>[3x]ARASPGSAASPRLREGPELSPDDPAGLLDLRQGMFAQLVAQNVLLIDGPLSWYSDPGLAGVSLTGGLSYKEDTKELVVAKAGVYYVFFQLELRRVVAGEGSGSVSLALHLQPLRSAAGAAALALTVDLPPASSEARNSAFGFQGRLLHLSAGQRLGVHLHTEARARHAWQLTQGATVLGLFRVTPEIPAGLPSPRSEGSHHHHHHHH;>[3x]QDPCSNCPAGTFCDNNRNQICSPCPPNSFS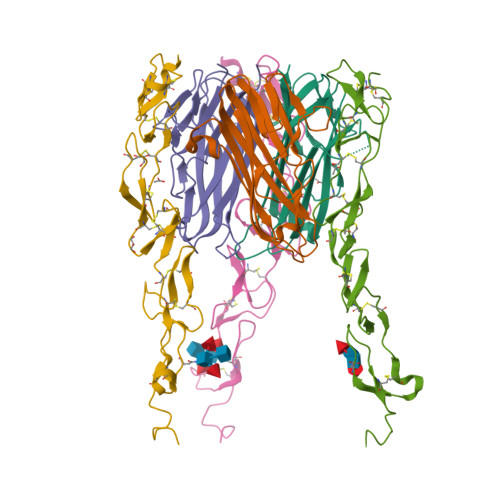SAGGQRTCDICRQCKGVFRTRKECSSTSNAECDCTPGFHCLGAGCSMCEQDCKQGQELTKKGCKDCCFGTFNDQKRGICRPWTNCSLDGKSVLVNGTKERDVVCGPSPENLYFQ>[2x]GAMDPSSPNYDKW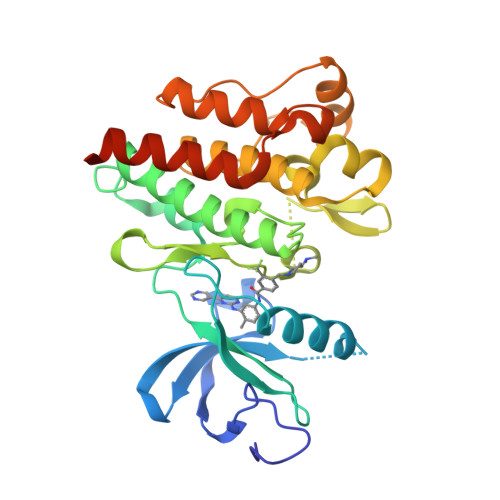EMERTDITMKHKLGGGQYGEVYEGVWKKYSLTVAVKTLKEDTMEVEEFLKEAAVMKEIKHPNLVQLLGVCTREPPFYIITEFMTYGNLLDYLRECNRQEVNAVVLLYMATQISSAMEYLEKKNFIHRDLAARNCLVGENHLVKVADFGLSRLMTGDTYTAHAGAKFPIKWTAPESLAYNKFSIKSDVWAFGVLLWEIATYGMSPYPGIDLSQVYELLEKDYRMERPEGCPEKVYELMRACWQWNPSDRPSFAEIHQAFETMFQESSISDEVEKELGKQGV>[4x]MSDSTPKTPRGFVVHTAPVGLADDGRDDFTVLASTAPATVSAVFTRSRFAGPSVVLCREAVADGQARGVVVLARNANVATGLEGEENAREVREAVARALGLPEGEM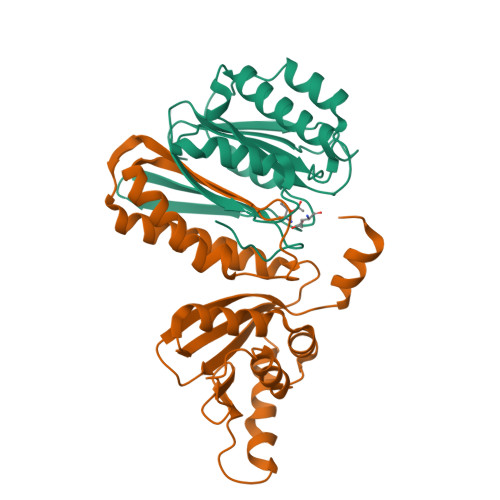LIASTGVIGRQYPMESIREHLKTLEWPAGEGGFDRAARAIMTTDTRPKEVRVSVGGATLVGIAKGVGMLEPDMA;>[4x]TLLTFFATDARLDPAEQDRLFRRVMDRTFNAVSIDTDTSTSDTAVLFANGLAGEVDAGEFEEALHTAALALVKDIASDGEGAAKLIEVQVTGARDDAQAKRVGKTVVNSPLVKTAVHGCDPNWGRVAMAIGKCSDDTDIDQERVTIRFGEVEVYPPKARGDQADDALRAAVAEHLRGDEVVIGIDLAIADGAFTVYGCDLTEGYVRLNSEYTT Cellvibrio japonicus is a saprotrophic bacterium which possesses the remarkable ability to grow in isolation using a variety of hemicellulosic polysaccharides as sole carbon sources. It produces a diverse collection of GHs, assembling enzyme systems that can degrade cellulose, xylans, mannans, and xyloglucans, among others. Effective xyloglucan-degrading GH systems (recently reviewed by Attia and Brumer) contain exo-acting glycosidases acting as debranching accessory enzymes and endo-acting enzymes (xyloglucanases) that generate short, branched β-(1,4)-glucan oligomers (xyloglucan oligosaccharides).18−23Exo-acting enzymes are expected to address each of the glycosidic linkages reported in xyloglucan branches, though the reported enzyme diversity falls short of reported branch diversity. The work presented here comprises the design and validation of trisaccharidic xyloglucan (“XyG”)-type cyclophellitol probes and their validation as bona fide, predictive tools for the identification of xyloglucanase activities and their discrimination from cellulase activities within a xyloglucan-elicited C. japonicus degradome.

Recombinant production and characterization of homology-selected putative xyloglucanases in the C. japonicus genome identified Cel5D, Cel5E, Cel5F, and CjGH74A as specific xyloglucanases, but the roles of each of these remain unclear. In order to validate the ABP-XyG probes for profiling xyloglucanases in complex biological samples, we first established the potency and mode of action of ABP-XyG-N3 as inhibitor of various previously characterized recombinant xyloglucanases. Incubation of pure recombinant Bacteroides ovatus BoGH5A,13Paenibacillus pabuli PpXG5,19 and C. japonicus CjCel5D with 100 μM ABP-XyG-N3 for 1 h under optimal activity conditions gave near-quantitative labeling as assessed by intact protein mass spectrometry analysis, while identical treatment with ABP-Cel-N3 gave minimal labeling. X-ray diffraction data of the complex between CjCel5D and ABP-XyG-N3 shows near-perfect mimicry of the known glycosyl enzyme intermediate state in the −1 and −2 subsites. Irreversible inhibition kinetics, measured using bespoke 4-methylumbelliferyl (4MU) and 6-chloro-4-methylumbelliferyl (6C4MU) XXXG fluorogenic substrates (see the Supporting Information for synthetic details and Tuomivaara et al. for oligosaccharide nomenclature), showed probe selectivity values ((ki,XyG-N3/KI,XyG-N3)/(ki,Cel-N3/KI,Cel-N3)) ranging from >17 for CjCel5D to 0.13 and <0.0026 for HiCel7B49 and BaCel5A,50 two well-known cellulases, respectively. We observed strong and uniquely xyloglucan-induced production of a ∼65 kDa ABP-XyG-Cy5-selective outer membrane-associated enzyme. Pulldowns from saturation cultures using ABP-βGlc-Bio, ABP-Cel-Bio, and ABP-XyG-Bio unambiguously identified Cel5D as the only exclusively ABP-XyG-Bio-reactive band, Cel5C as the exclusively ABP-Cel-Bio-reactive band, and Cel3A, Cel3B, and Cel3D as the ABP-βGlc-reactive bands.

> MGSSHHHHHHSSGLVPRGSHMASGLYPSYNTSPAAPDSTGMQSTAVQLAGKIRLGWNIGNTMEAIGGETAWGNPMVSNELLKLVKDSGFDAVRIPVAWDQYANQESAEISAAWLNRVKQVVQMAIDNELYVLINIHWDGGWLENNITPAKKDENNAKQKAFWEQIATHLRDFDEHLLFAGTNEPNAENAEQMDVLNSYLQTFVDAVRSTGGKNAYRVLVLQGPVTDIEKTNELWTHMPADTATDRLMAEVHFYTPYNFALMRQDESWGKQFYYWGEGFLSTTDTERNPTWGEEATIDQLFDLMKTKFVDQGIPVVLGEFSAMRRTNLTGDALTLHLAGRAYYHKYVTQQALARGLLPFYWDNGGNDNFSSGIFNRQQNTVFDQQVLDALLEGAGAQ> MSEDD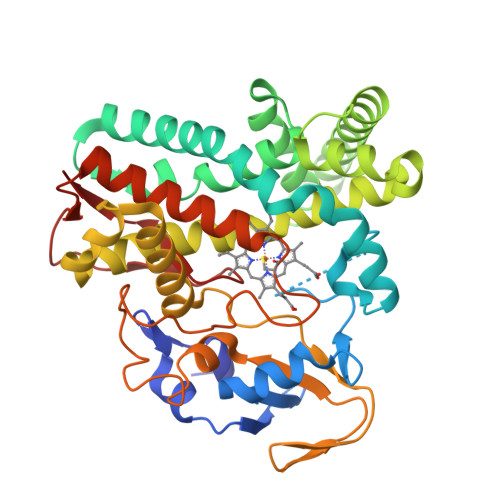PRPLHIRRQGLDPADELLAAGALTRVTIGSGADAETHWMATAHAVVRQVMGDHQQFSTRRRWDPRDEIGGKGIFRPRELVGNLMDYDPPEHTRLRRKLTPGFTLRKMQRMAPYIEQIVNDRLDEMERAGSPADLIAFVADKVPGAVLCELVGVPRDDRDMFMKLCHGHLDASLSQKRRAALGDKFSRYLLAMIARERKEPGEGMIGAVVAEYGDDATDEELRGFCVQVMLAGDDNISGMIGLGVLAMLRHPEQIDAFRGDEQSAQRAVDELIRYLTVPYSPTPRIAREDLTLAGQEIKKGDSVICSLPAANRDPALAPDVDRLDVTREPIPHVAFGHGVHHCLGAALARLELRTVFTELWRRFPALRLADPAQDTEFRLTTPAYGLTELMVAW>[4x]SNANRDSLFNDPNAPVLGNPEGDVTVVEFFDYNCPY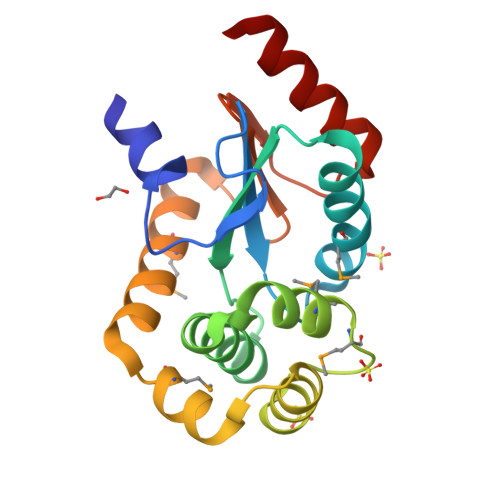CRRAMAEVQGLVDADPNVRLVYREWPILGEGSDFAARAALAARQQGKYEAFHWALMGMSGKANETGVLRIAREVGLDTEQLQRDMEAPEVTAHIAQSMALAQKLGFNGTPSFVVEDALVPGFVEQSQLQDAVDRARKAA>[2x]GPMIDTFSRTGPLMEAASYPAWTQQLIQDCSESKRRVVEHELYQRMRDNKLSAKVMRQYLIGGWPVVEQFALYMAQNLTKTRFARHPGEDMARRWLMRNIRVELNH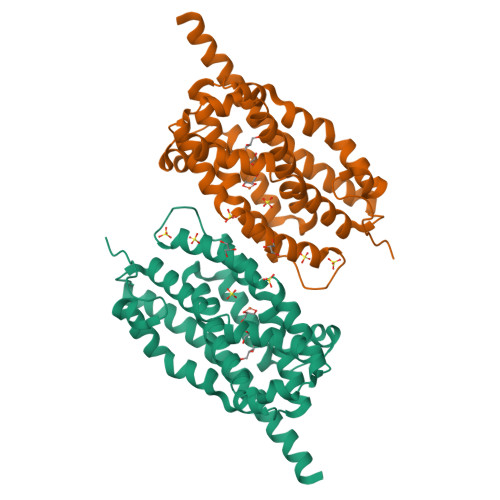ADYWVHWSRAHGVTLEDLQAQQVPPELHALSHWCWHTSSADSLIVAIAATNYAIEGATGEWSALVCSNGIYAAAFPEEDRKRAMKWLKMHAQYDDAHPWEALEIIVTLAGLNPTKALQAELRQAICKSYDYMYLFLERCMQQEKTAVTRERLALAEG>MHHHHHHGSMIQKRKTRQIRVGNVKIGGDAPIVVQSMTSTKTHDVEATLNQIKRLYEAGCEIVRVAVPHKEDVEALEEIVKKSPMPVIADIHFAPSYAFLSMEKGVHGIRINPGNIGKEEIVREIVEEAKRRGVAVRIGVNSGSLEKDLLEKYGYPSAEALAESALRWSEKFEKWGFTNYKVSIKGSDVLQNVRANLIFAERTDVPLHIGITEAGMGTKGIIKSSVGIGILLYMGIGDT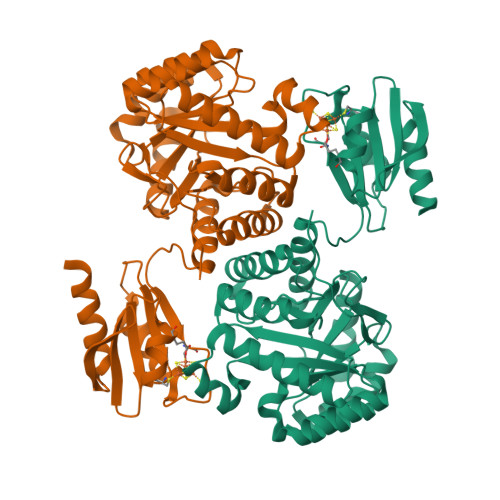VRVSLTDDPVVEVETAYEILKSLGLRRRGVEIVACPTCGRIEVDLPKVVKEVQEKLSGVKTPLKVAVMGCVVNAIGEAREADIGLACGRGFAWLFKHGKPIKKVDESEMVDELLKEIQNMEKDGGTN[4x]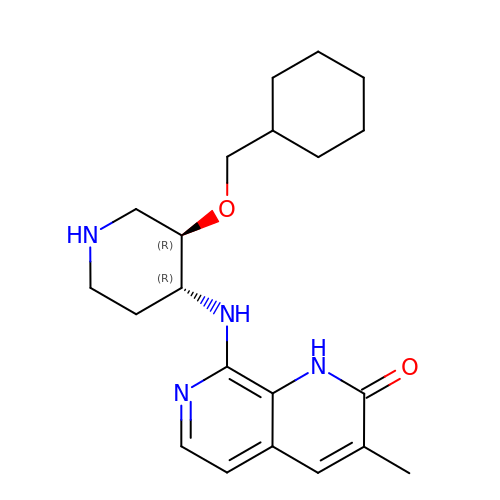(3R,4R)-3-(cyclohexylmethoxy)piperidin-4-yl]amino}-3-methyl-1,2-dihydro-1,7-naphthyridin-2-one | C21 H30 N4 O2 | DQJOFVKRLCBKNO-QZTJIDSGSA-N>[3x]GSHMSAPLPLDELRTFAEVLDRVKAAYVEPVDDKTLLENAIKGMLSNLDPHS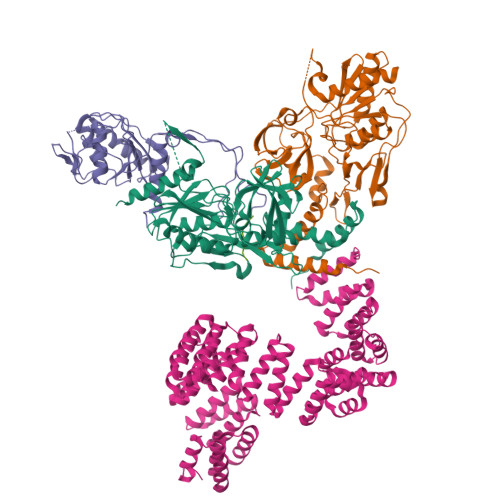AYLGPEDFAELQESTSGEFGGLGIEVGSEDGFIKVVSPIDDTPAARAGIQPGDLIVQIDGKPTKGQSMTEAVDSMRGKAGSPITLTIVRDGGRPFDVELKRAIIKVKSVKSQVLEPGYAYLRITQFQVNTGEEVVKALNQLRKDNKGRLKGLVLDLRNNPGGVLQSAVEVADAFLTKGLIVYTKGRIANSELRFSADPADPSDKVPLVVLINGGSAAAAEIVAGALQDQKRAILMGTDSFGKGSVQTVLPLNNDRALKLTTALYYTPNGRSIQAQGIVPDIEVGRAKVTQERSSFEGFKEADLQGHLANGNGGADRPTGKRAAPSERPQDSDYQLSQALSLLKGLSVTRGN;> MEDTAVETKAKPEKYGSFSEDSLYSLLVAELAGQRNRFDIALSNYVVQAQKTRDPGVSERAFRIAEYLGADQEALDTSLLWARSAPDNLDAQRAAAIQLARAGRYEESMVYMEKVLNGQGDTHFDFLALSAAETDPDTRAGLLQSFDHLLKKYPNNGQLLFGKALLLQQDGRPDEALTLLEDNSASRHEVAPLLLRSRLLQSMKRSDEALPLLKAGIKEHPDDKRVRLAYARLLVEQNRLDDAKAEFAGLVQQFPDDDDLRFSLALVCLEAQAWDEARIYLEELVERDSHVDAAHFNLGRLAEEQKDTARALDEYAQVGPGNDFLPAQLRQTDVLLKAGRVDEAAQRLDKARSEQPDYAIQLYLIEAEALSNNDQQEKAWQAIQEGLKQYPEDLNLLYTRSMLAEKRNDLAQMEKDLRFVIAREPDNAMALNALGYTLADRTTRYGEARELILKAHKLNPDDPAILDSMGWINYRQGKLADAERYLRQALQRYPDHEVAAHLGEVLWAQGRQGDARAIWREYLDKQPDSDVLRRTIKRLTGAETP>[2x]SNALENMYHLFQLKRETDDLEQWISEKELVASSPEMGQDFDHVTLLRDKFRDFARETGAIGQERVDNVNAFIERLIDAGHSEAATIAEWK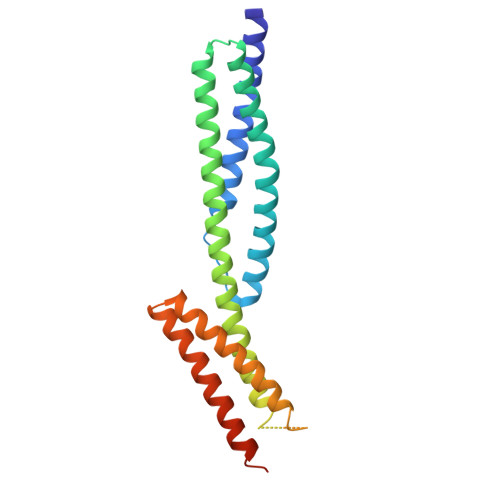DGLNEMWADLLELIDTRMQLLAASYDLHRYFYTGAEILGLIDEKHRELPEDVGLDASTAESFHRVHTAFERDVHLLGVQVQQFQDVATRLQTAYAGEKAEAIQNKEQEVSAAWQALLDACAGRRTQLVDTADKFR8-{[2-(dimethylamino)ethyl]amino}-3-methyl-1,2-dihydroquinolin-2-one | C14 H19 N3 O | 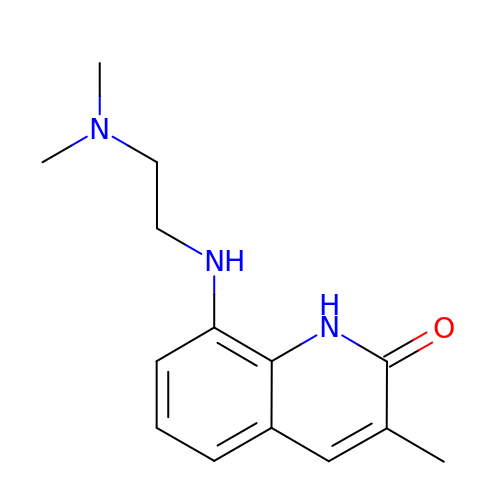RIMSJTCQEYACPJ-UHFFFAOYSA-N> MNNSEDPFQQVVKDTKEQLNRINNYITRH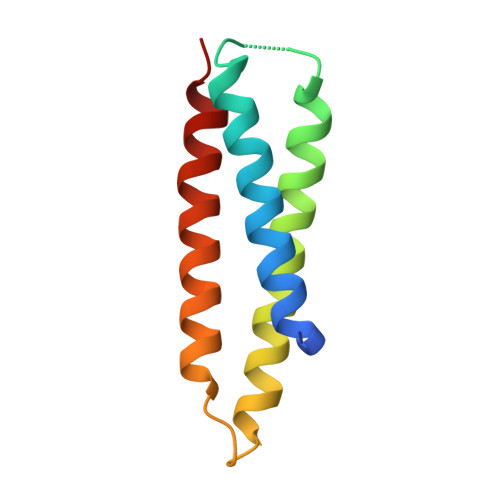NTAGDDDQEEEIQDILKDVEETIVDLDRSIIVMKRDENEDVSGREAQVKNIKQQLDALKLRFDRRI>[12x]GDELYRQSLEIISR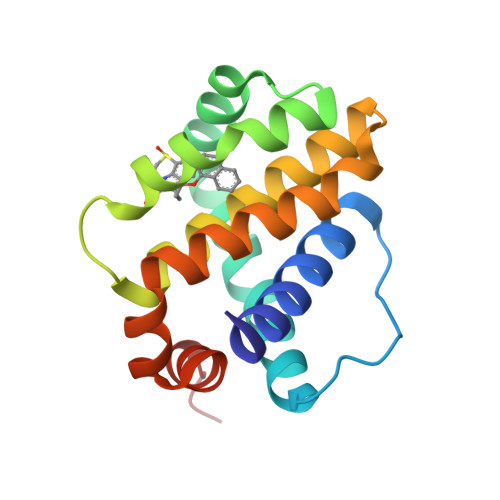YLREQATGAKDTKPMGRSGATSRKALETLRRVGDGVQRNHETAFQGMLRKLDIKNEDDVKSLSRVMIHVFSDGVTNWGRIVTLISFGAFVAKHLKTINQESCIEPLAESITDVLVRTKRDWLVKQRGWDGFVEFFHVEDLEGG> MTIDQKNTNIDPRFPHHHPRPQSFWEARAKALESLLIEKGHLSSDAIERVIKHYEHELGPMNGAKVVAKAWTDPAFKQRLLEDSETVLRELGYYGLQGEHIRVVENTDTVHNVVVCTLCSCYPWPLLGLPPSWYKEPAYRARVVKEPRQVLKEFGLDLPDSVEIRVWDRSSEIRFMVLPQRPEGTEGMTEEELAKLVTRDSMIGVAKIEPP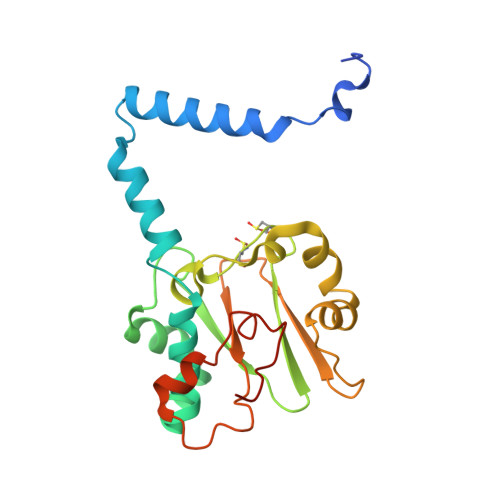KVTVG>[2x]HEHNTIPKGASIEVKVQQLDPVNGNKDVGTVTITESNYGLVF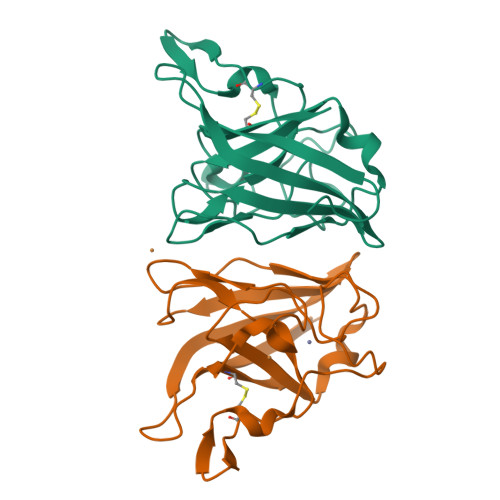TPDLQGLSEGLHGFHIHENPSCEPKEEEGELTAGLGAGGHWDPKGAKQHGYPWQDDAHLGDLPALTVLHDGTATNPVLAPRLKHLDDVRGHSIMIHTGGDNHSDHPAPLGGGGPRMACGVIK>[3x]VKTPGTRYVTHKQLDEKLKNFVTKTEFKEFQTVVMESFAVQNQNIDAQGEQIK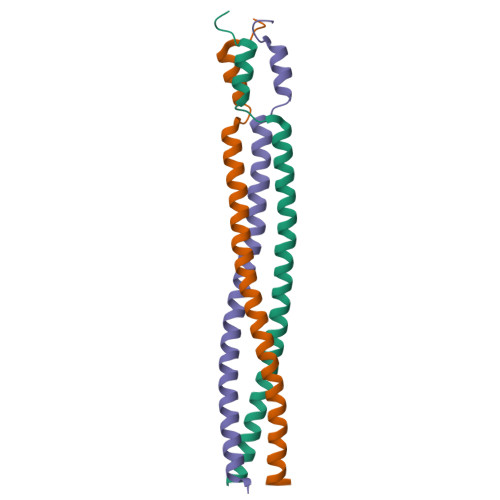ELQVEQKAQGKTLQLILEALQGINKRLDNLES>GHMELKREEITLLKELGSGQFGVVKLGKWKGQYDVAVKMIKEGSMSEDEFFQEAQTMMKLSHPKLVKFYGVCSKEYPIYIVTEYISNGCLLNYLRSHGKGLEPSQLLEMCYDVCEGMAFLESHQFIHR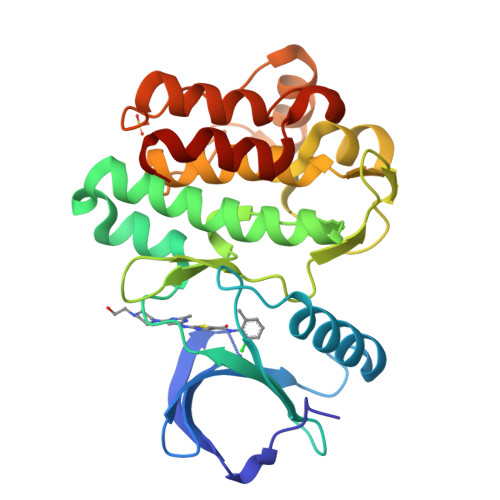DLAARNCLVDRDLCVKVSDFGMTRYVLDDQYVSSVGTKFPVKWSAPEVFHYFKYSSKSDVWAFGILMWEVFSLGKMPYDLYTNSEVVLKVSQGHRLYRPHLASDTIYQIMYSCWHELPEKRPTFQQLLSSIEPLREKDKH[2x]> MKRLSSHHAIVCGAASATAASTRFGDVVGGGSSCTATSPLFAAQRGRFYRPLVNQGINLWRSRMGRLHKGWTTWEYNRDVIPDPRPFPEPAVNNYFGRSRIWNPIAGKIGLVNRKAEEWGWPHQRPPPTGLRRSPEYFPFF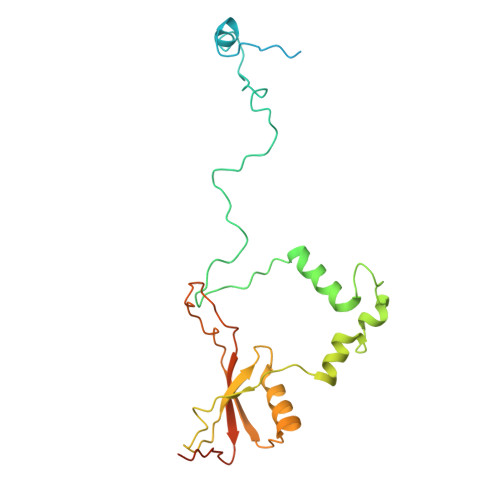FSRYFPDVEVRLVLDSVLNNETTRPIFHIPQDMSKQELVNYLKNIYNIDNVVRIRVRNMRGRRFKNEVGEIKSLPDYKVAVVELDSPVSIVFKQIKGTEDTPDNKPAAQIT>LEEKKVCQGTSNKLTQLGTFEDHFLSLQRMFNNCEVVLGNLEITYVQRNYDLSFLKTIQEVAGYVLIALNTVERIPLENLQIIRGNMYYENSYALAVLSNYDANKTGLKELPMRNLQEILHGAVRFSNNPALCNVESIQWRDIVSSDFLSNMSMDFQNHLGSCQKCDPSCPNGSCWGAGEENCQKLTKIICAQQCSGRCRGKSPSDCCHNQCAAGCTGPRESDCLVCRKFRDEATCKDTCPPLMLYNPTTYQMDVNPEGKYSFGVTCVKKCPRNYVVTDHGSCVRACGADSYEMEEDGVRKCKKCEGPCRKVCNGIGIGEFKDSLSI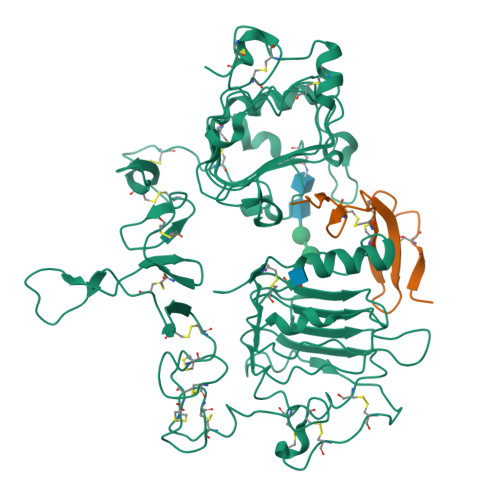NATNIKHFKNCTSISGDLHILPVAFRGDSFTHTPPLDPQELDILKTVKEITGFLLIQAWPENRTDLHAFENLEIIRGRTKQHGQFSLAVVSLNITSLGLRSLKEISDGDVIISGNKNLCYANTINWKKLFGTSGQKTKIISNRGENSCKATGQVCHALCSPEGCWGPEPRDCVSHHHHHH[4x];>VSITKCSSDMNGYCLHGQCIYLVDMSQNYCRCEVGYTGVRCEHFFLTV[4x]>[2x]M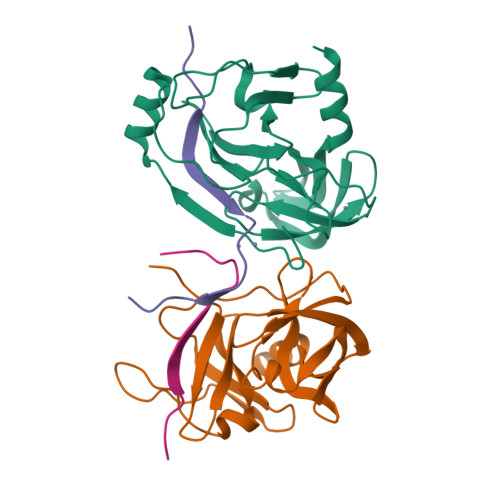ASMTGGQQMGAPITAYAQQTRGLLGCIITSLTGRDKNQVEGEVQIVSTATQTFLATCINGVCWTVYHGAGTRTIASPKGPVIQMYTNVDQDLVGWPAPQGSRSLTPCTCGSSDLYLVTRHADVIPVRRRGDSRGSLLSPRPISYLKGSAGGPLLCPAGHAVGLFRAAVCTRGVAKAVDFIPVENLETTMRSGSHHHHHH;>KKGCVVIVGRIVLSGKPAIIPKK[2x]> MATPDQKSPNVLLQNLCCRILGKSEADVAQQFQYAVRVIGSNFAPTVERDEFLVAEKIKKELTRQRREADAALFSELHRKLHSQGVLKNKWSILYLLLSLSEDPRKQPSKVSGYAALFAQALPRDAHSTPYYYARPQSLPLNYQERGAPSAQSAGSAGSSGVSSLGTYALNGPTPPPPPPALLPGQPLPAPGVGDGLRQQLGSRLAWTLTASQPSLPSTTSKAVPSSGSRGAARPRREGDAAAGAVEVTEAALVRDILYVFQGIDGKHVKMSNADNCYTVEGKANLSKSLRDTAVRLAELGWLHNKIRKYTDQRSLDRSFGLVGQSFCAALHQELREYYRLLSVLHSQLQLEDDQGVNLGLESSLTLRRLLVWTYDPKMRLKTLAALVDHCQGRKGGELASAVHAYTKTGDPYARSLVQHILSLVSHPVLSFLYRWIYDGELEDTYHEFFVASDPAVKADRLWHDKYALRKPMIPSFMTMDQCRKVLLIGKSINFLHQVCHDQTPTTKMIAVTKSAESPQDAADLFTDLENAFQGKIDAAYFETSKYLLDVLNKKYSLLDHMQAMRRYLLLGQGDFIRHLMDLLKPELVRPATTLYQHNLTGILETAVRATNAQFDSPEILKRLDVRLLEVSPGDTGWDVFSLDYHVDGPIATVFTRECMSHYLRAFNFLWRAKRVEYILTDIRKGHMCNARLLRSMPEFSGVLHHCHILASEMVHFIHQMQYYVTFEVLECSWDELWNRVQRAQDLDHIIAAHEAFLGTVISRCLLDSDSRALLNQLRAVFDQIIELQNTQDAIYRAALEELQRRLQFEEKKKQREAEGQWGVSAAEEEQEKRRVQEFQESIPKMCSQLRILTHFYQGVVQQFLVSLTTSSDESLRFLSFRLDFNEHYRAREPRLRVSLGTRGRRSSHT;> MSEFRIHHDVNELLSLLRVHGGDGAEVYIDLLQKNRTPYVTTTVSAHSAKVKIAEFSRTPEDFLKKYDELKSKNTRNLDPLVYLLSKLMEDRETLQYLQQNAKERAELAASAAASSTASFG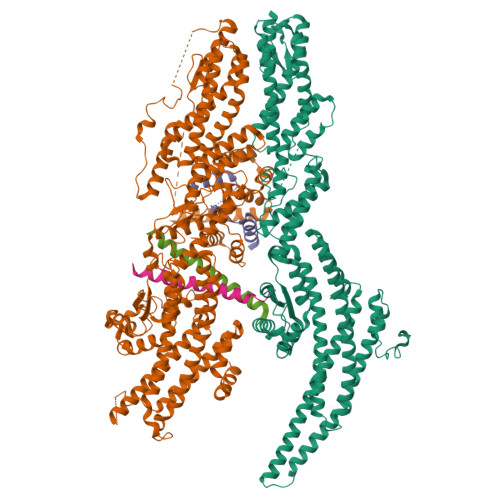ASATASKISMQELEELRKQLGSVATGPTWQQSLELTRKMLRDKQSKKNSGQRLPVLPAWVYERPALLGDFLPGTGGSADTAVPIGSLPLASQEAAVVEDLLYVLVGVDGRYISAQPLTGRQGRTFLVDPNLDLSIRELVSRILPVAASYSTVTRFIEEKSSFEYGQVNHALAAAMRTLVKEYLVLVTQLEQLQRQGLLSLQKLWFYIQPAMRSLDILASLATSVDKGECIGGATLSLLHDRSFSYTGDSQAQELCLHLTKAASTPYFEILEKWIYRGIIDDPYSEFMVEEHELRKEKIQEDYNDKYWDQRYTVVQRQIPSFLQKMAGKVLSTGKYLNVVRECGHDVTCPVAKEVVYTLKERAYVEQIEKAFSYASKVLLDFLMGEKELLAHLRSIKRYFLMDQGDFFVHFMDLTEEELKKPVDDITPTRLEALLELALRMSTANTDPFKDDLKIDLMPHDLITQLLRVLAIETQQEKAMVHADPTELTLSGLEAFSFDYVVTWPLSLIINRKALTRYQMLFRHMFYCKHVERQLCSVWISNKAAKRFSLHSAKWFAGAFTLRQRMLNFVQNIQSYMMFEVMEPTWHVLEQNLRSASNIDDVLGHHASFLDNCLKDCMLTNPELLRVFSKLMSVCVMFTNCLQRFTQSMKLDSELGHPALEPGAMLGPPTEAERAEERARKELARKCLAEHVDAPQLASSFEATITKFDKNFSAHLLDLLARLSIYSTSDCEHGMASVISRLDFNGFYTERLERLSAERSQKAAPPVPGPRGPPALVPRVAVTAQ;> MAAPGAGPGPGAPPGLEAALQKLALRRKKVLSAEETELFELAQAAGGAMDPEVFKILVDLLKLNVAPLAVFQMLKSMCAGQRLASEPQDPVAVPLPTTSVPETRGRNRGSSALGGGPALAERSGREGSSQRMPRQPSATRLPKGGGPGKSPTRST;>[2x]MMDLVLEEDVTVPGTLSGCSGLVPSVPDDLDGINPNAGLGNGLLPNVSEETVSPTRARNMKDFENQITELKKENFNLKLRIYFLEERMQQEFHGPTEHIYKTNIELKVEVESLKRELQEREQLLIKASKAVESLAEAGGSEIQRVKEDARKKVQQVEDLLTKRILLLEKDVTAAQAELEKAFAGTETEKALRLRLESKLSEMKKMHEGDLAMALVLDEKDRLIEELKLSLKSKEALIQCLKEEKSQMACPDENVSSGELRGLCAAPREEKERETEAAQMEHQKERNSFEERIQALEEDLREKEREIATEKKNSLKRDKAIQGLTMALKSKEKKVEELNSEIEKLSAAFAKAREALQKAQTQEFQGSEDYETALSGKEALSAALRSQNLTKSTENHRLRRSIKKITQELSDLQQERERLEKDLEEAHREKSKGDCTIRDLRNEVEKLRNEVNEREKAMENRYKSLLSESNKKLHNQEQVIKHLTESTNQKDVLLQKFNEKDLEVIQQNCYLMAAEDLELRSEGLITEKCSSQQPPGSKTIFSKEKKQSSDYEELIQVLKKEQDIYTHLVKSLQESDSINNLQAELNKIFALRKQLEQDVLSYQNLRKTLEEQISEIRRREEESFSLYSDQTSYLSICLEENNRFQVEHFSQEELKKKVSDLIQLVKELYTDNQHLKKTIFDLSCMGFQGNGFPDRLASTEQTELLASKEDEDTIKIGEDDEINFLSDQHLQQSNEIMKDLSKGGCKNGYLRHTESKISDCDGAHAPGCLEEGAFINLLAPLFNEKATLLLESRPDLLKVVRELLLGQLFLTEQEVSGEHLDGKTEKTPKQKGELVHFVQTNSFSKPHDELKLSCEAQLVKAGEVPKVGLKDASVQTVATEGDLLRFKHEATREAWEEKPINTALSAEHRPENLHGVPGWQAALLSLPGITNREAKKSRLPILIKPSRSLGNMYRLPATQEVVTQLQSQILELQGELKEFKTCNKQLHQKLILAEAVMEGRPTPDKTLLNAQPPVGAAYQDSPGEQKGIKTTSSVWRDKEMDSDQQRSYEIDSEICPPDDLASLPSCKENPEDVLSPTSVATYLSSKSQPSAKVSVMGTDQSESINTSNETEYLKQKIHDLETELEGYQNFIFQLQKHSQCSEAIITVLCGTEGAQDGLSKPKNGSDGEEMTFSSLHQVRYVKHVKILGPLAPEMIDSRVLENLKQQLEEQEYKLQKEQNLNMQLFSEIHNLQNKFRDLSPPRYDSLVQSQARELSLQRQQIKDGHGICVISRQHMNTMIKAFEELLQASDVDYCVAEGFQEQLNQCAELLEKLEKLFLNGKSVGVEMNTQNELMERIEEDNLTYQHLLPESPEPSASHALSDYETSEKSFFSRDQKQDNETEKTSVMVNSFSQDLLMEHIQEIRTLRKRLEESIKTNEKLRKQLERQGSEFVQGSTSIFASGSELHSSLTSEIHFLRKQNQALNAMLIKGSRDKQKENDKLRESLSRKTVSLEHLQREYASVKEENERLQKEGSEKERHNQQLIQEVRCSGQELSRVQEEVKLRQQLLSQNDKLLQSLRVELKAYEKLDEEHRRLREASGEGWKGQDPFRDLHSLLMEIQALRLQLERSIETSSTLQSRLKEQLARGAEKAQEGALTLAVQAVSIPEVPLQPDKHDGDKYPMESDNSFDLFDSSQAVTPKSVSETPPLSGNDTDSLSCDSGSSATSTPCVSRLVTGHHLWASKNGRHVLGLIEDYEALLKQISQGQRLLAEMDIQTQEAPSSTSQELGTKGPHPAPLSKFVSSVSTAKLTLEEAYRRLKLLWRVSLPEDGQCPLHCEQIGEMKAEVTKLHKKLFEQEKKLQNTMKLLQLSKRQEKVIFDQLVVTHKILRKARGNLELRPGGAHPGTCSPSRPGS>MIPVTELRYFADTQPAYRILKPWWDVFTDYISIVMLMIAVFGGTLQVTQDKMICLPCKWVTKDSCNDSFRGWAASSPEPTYPNSTVLPTPDTGPTGIKYDLDRHQYNYVDAVCYENRLHWFAKYFPYLVLLHTLIFLACSNFWFKFPRTSSKLEHFVSILLKCFDSPWTTRALSETVVEESDPKPAFSKMNGSMDKKSSTVSEDVEATVPMLQRTKSRIEQGIVDRSETGVLDKKEGEQAKALFEKVKKFRTHVEEGDIVYRLYMRQTIIKVIKFALIICYTVYYVHNIKFDVDC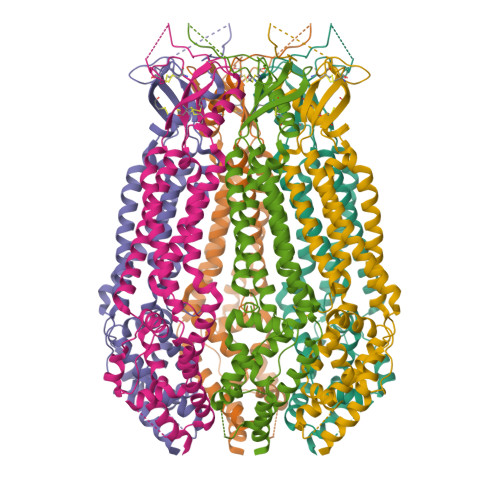TVDIESLTGYRTYRCAHPLATLFKILASFYISLVIFYGLICMYTLWWMLRRSLKKYSFESIREESSYSDIPDVKNDFAFMLHLIDQYDPLYSKRFAVFLSEVSENKLRQLNLNNEWTLDKLRQRLTKNAQDKLELHLFMLSGIPDTVFDLVELEVLKLELIPDVTIPPSIAQLTGLKELWLYHTAAKIEAPALAFLRENLRALHIKFTDIKEIPLWIYSLKTLEELHLTGNLSAENNRYIVIDGLRELKRLKVLRLKSNLSKLPQVVTDVGVHLQKLSINNEGTKLIVLNSLKKMVNLTELELIRCDLERIPHSIFSLHNLQEIDLKDNNLKTIEEIISFQHLHRLTCLKLWYNHIAYIPIQIGNLTNLERLYLNRNKIEKIPTQLFYCRKLRYLDLSHNNLTFLPADIGLLQNLQNLAVTANRIEALPPELFQCRKLRALHLGNNVLQSLPSRVGELTNLTQIELRGNRLECLPVELGECPLLKRSGLVVEEDLFSTLPPEVKERLWRADKEQA[6x]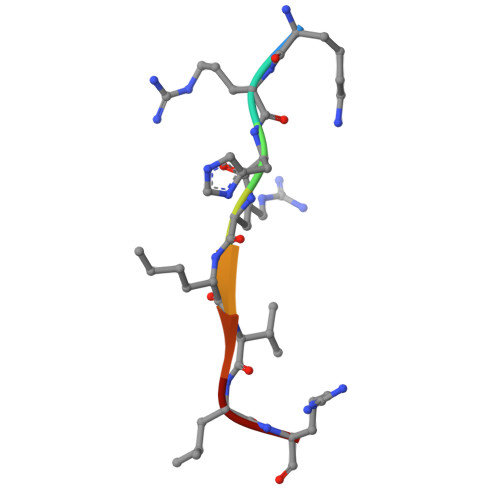> KRHRLVLR5-(4-fluorophenyl)-~{N}-[[3-[(~{R})-(1-methylindazol-5-yl)-oxidanyl-methyl]phenyl]methyl]-2,3-bis(oxidanyl)benzamide | C29 H24 F N3 O4 | 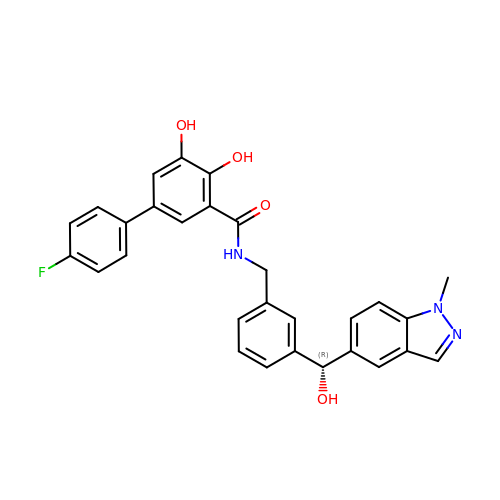AYTCJOWSEKPFCS-HHHXNRCGSA-N>GSHGMKVVIAGRPNAGKSSLLNALAGREAAIVTDIAGTTRDVLREHIHIDGMPLHIIDTAGLREASDEVERIGIERAWQEIEQADRVLFMVDGTTTDAVDPAEIWPEFIARLPAKLPITVVRNKADITGETLGMSEVNGHALIRLSARTGEGVDVLRNHL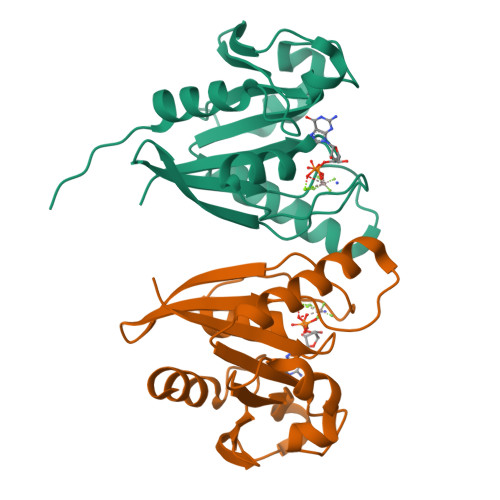KQSMGFDTNMEG[2x]>MGSVRTNRYSIVSSEEDGMKLATMAVANGFGNGKSKVHTRQQCRSRFVKKDGHCNVQFINVGEKGQRYLADIFTTCVDIRWRWMLVIFCLAFVLSWLFFGCVFWLIALLHGDLDASKEGKACVSEVNSFTAAFLFSIETQTTIGYGFRCVTDECPIAVFMVVFQSIVGCIIDAFIIGAVMAKMAKPKKRNETLVFSHNAVIAMRDGKLCLMWRVGNLRKSHLVEAHVRAQLLKSRITSEGEYIPLDQIDINVGFDSGIDRIFLVSPITIVHEIDEDSPLYDLSKQDIDNADFEIV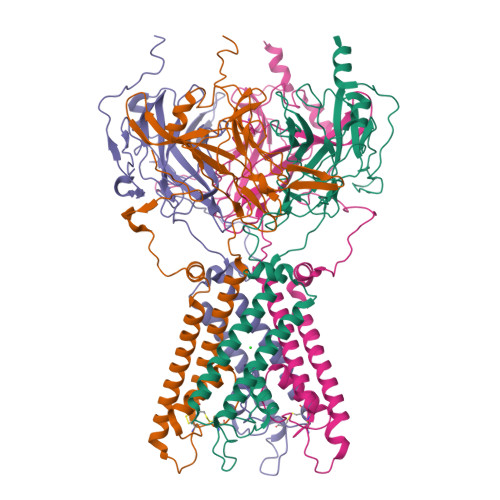VILEGMVEATAMTTQCRSSYLANEILWGHRYEPVLFEEKHYYKVDYSRFHKTYEVPNTPLCSARDLAEKKYILSNANSFCYENEVALTSKEEDDSENGVPESTSTDTPPDIDLHNQASVPLEPRPLRRESEI[4x]(4E)-4-{3-[(4-amino-2-methylpyrimidin-5-yl)methyl]-5-(2-{[(S)-hydroxy(phosphonooxy)phosphoryl]oxy}ethyl)-4-methyl-1,3-thiazol-2(3H)-ylidene}-4-hydroxybutanoic acid | C16 H24 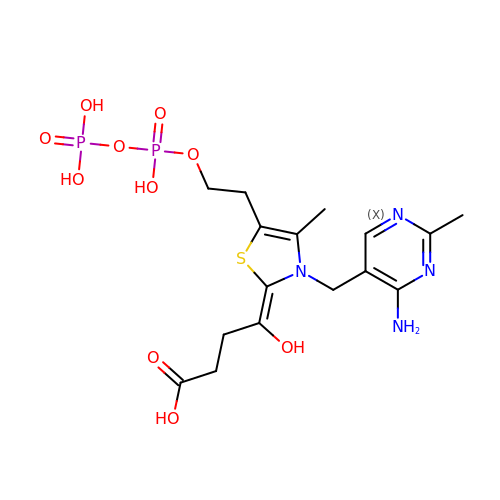N4 O10 P2 S | VGWJMSNWDAXPBE-FOWTUZBSSA-N>[4x]SYTLPSLPYAYDALE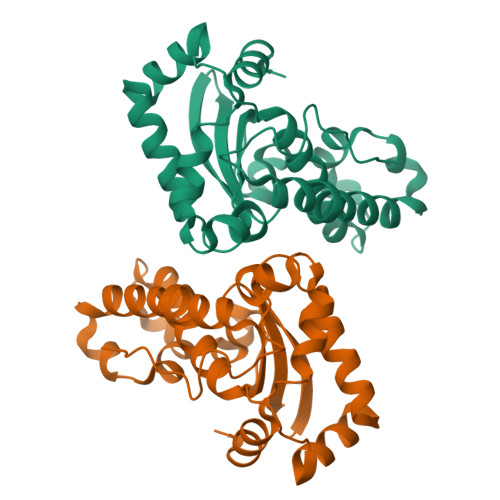PHFDKQTMEIHHTKHHQTYVNNANAALESLPEFANLPVEELITKLDQLPADKKTVLRNNAGGHANHSLFWKGLKKGTTLQGDLKAAIERDFGSVDNFKAEFEKAAASRFGSGWAWLVLKGDKLAVVSTANHDSPLMGEAISGASGFPIMGLDVWEHAYYLKFQNRRPDYIKEFWNVVNWDEAAARFAAKK> MYTMGLDIGSTASKGVILKNGEDIVASETISSGTGTTGPSRVLEKLYGKTGLAREDIKKVVVTGYGRMNYSDADKQISELSCHARGVNFIIPETRTIIDIGGQDAKVLKLDNNGRLLNFLMNDKCAAGTGRFLDVMAKIIEVDVSELGSISMNSQNEVSISSTCTVFAESEVISHLSENAKIEDIVAGIHTSVAKRVSSLVKRIGVQRNVVMVGGVARNSGIVRAMAREINTEIIVPDIPQLTGALGAALYAFDEAKESQKEVKNISAWS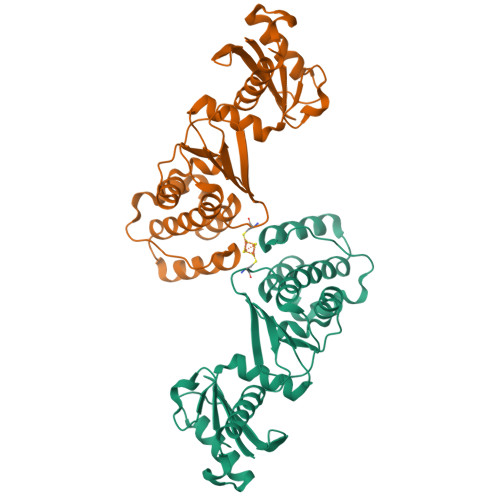HPQFEK> MNDDRETPPKRKPGEDDTLFDIDFLDDTTSHSGSRSKVTNSHANANYIPPSHVLPEETIDLDADDDNIENDVHENLFMSNNHDDQTSWNANRFDSDAYQPQSLRAVKPPGLFARFGNGLKNAFTFKRKKGPESFEMNHYNAVTNNELDDNYLDSRNKFNIKILFNRYILRKNVGDAEGNGEPRVIHINDSLANSSFGYSDNHISTTKYNFATFLPKFLFQEFSKYANLFFLCTSAIQQVPHVSPTNRYTTIGTLLVVLIVSAMKECIEDIKRANSDKELNNSTAEIFSEAHDDFVEKRWIDIRVGDIIRVKSEEPIPADTIILSSSEPEGLCYIETANLDGETNLKIKQSRVETAKFIDVKTLKNMNGKVVSEQPNSSLYTYEGTMTLNDRQIPLSPDQMILRGATLRNTAWIFGLVIFTGHETKLLRNATATPIKRTAVEKIINRQIIALFTVLIVLILISSIGNVIMSTADAKHLSYLYLEGTNKAGLFFKDFLTFWILFSNLVPISLFVTVELIKYYQAFMIGSDLDLYYEKTDTPTVVRTSSLVEELGQIEYIFSDKTGTLTRNIMEFKSCSIAGHCYIDKIPEDKTATVEDGIEVGYRKFDDLKKKLNDPSDEDSPIINDFLTLLATCHTVIPEFQSDGSIKYQAASPDEGALVQGGADLGYKFIIRKPNSVTVLLEETGEEKEYQLLNICEFNSTRKRMSAIFRFPDGSIKLFCKGADTVILERLDDEANQYVEATMRHLEDYASEGLRTLCLAMRDISEGEYEEWNSIYNEAATTLDNRAEKLDEAANLIEKNLILIGATAIEDKLQDGVPETIHTLQEAGIKIWVLTGDRQETAINIGMSCRLLSEDMNLLIINEETRDDTERNLLEKINALNEHQLSTHDMNTLALVIDGKSLGFALEPELEDYLLTVAKLCKAVICCRVSPLQKALVVKMVKRKSSSLLLAIGDGANDVSMIQAAHVGVGISGMEGMQAARSADIAVGQFKFLKKLLLVHGSWSYQRISVAILYSFYKNTALYMTQFWYVFANAFSGQSIMESWTMSFYNLFFTVWPPFVIGVFDQFVSSRLLERYPQLYKLGQKGQFFSVYIFWGWIINGFFHSAIVFIGTILIYRYGFALNMHGELADHWSWGVTVYTTSVIIVLGKAALVTNQWTKFTLIAIPGSLLFWLIFFPIYASIFPHANISREYYGVVKHTYGSGVFWLTLIVLPIFALVRDFLWKYYKRMYEPETYHVIQEMQKYNISDSRPHVQQFQNAIRKVRQVQRMKKQRGFAFSQAEEGGQEKIVRMYDTTQKRGKYGELQDASANPFNDNNGLGSNDFESAEPFIENPFADGNQNSNRFSSSRDDISFDIGGGGLVPRG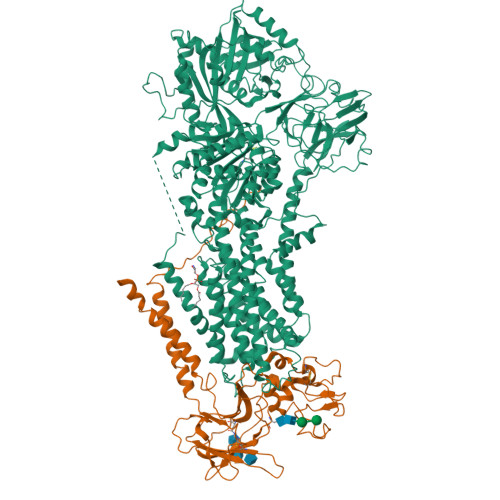SGGTAAAPGPAPAPAPASAPAAAAPAGAGTPVTAPLAGTIWKVLASEGQTVAAGEVLLILEAMKMETEIRAAQAGTVRGIAVKAGDAVAVGDTLMT;> MVSLFKRGKAPPLTKEGPTSKKPPNTAFRQQRLKAWQPILSPQSVLPLLIFVACIFTPIGIGLIVSATKVQDLTIDYSHCDTKASTTAFEDIPKKYIKYHFKSKVENKPQWRLTENENGEQSCELQFEIPNDIKKSIFIYYKITNFYQNHRRYVQSFDTKQILGEPIKKDDLDTSCSPIRSREDKIIYPCGLIANSMFNDTFSQVLSGIDDTEDYNLTNKHISWSIDRHRFKTTKYNASDIVPPPNWMKKYPDGYTDENLPDIHTWEEFQVWMRTAAFPKFYKLTLKNESASLPKGKYQMNIELNYPISLFGGTKSFVLTTNGAIGGRNMSLGVLYLIVAGLCALFGIIFLVKLIFQPRAMGDHTYLNFDDEENEDYEDVHAENTTLREILGGGGLVPRGSGGHHHHHHHHHH>MIVSAIAANALLESVTKFHCGVIYDYSTAEYVSYRPSDFGAYLDALEAEVARGGLIVFHNGHKYDVPALTKLAKLQLNREFHLPRENCIDTLVLSRLIHSNLKDTDMGLLRSGKLPGKRFGSHALEAWGYRLGEMKGEYKDDFKRMLEEQGEEYVDGMEWWNFNEEMMDYNVQDVVVTKALLEKLLSDKHYFPPEIDFTDVGYTTFWSESLEAVDIEHRAAWLLAKQERNGFPFDTKAIEELYVELAARRSELLRKLTETFGSWYQPKGGTEMFCHPRTGKPLPKYPRIKTPKVGGIFKKPKNKAQREGREPCELDTREYVAGAPYTPVEHVVFNPSSRDH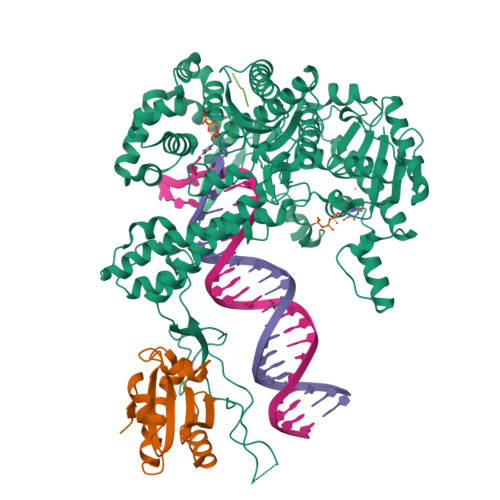IQKKLQEAGWVPTKYTDKGAPVVDDEVLEGVRVDDPEKQAAIDLIKEYLMIQKRIGQSAEGDKAWLRYVAEDGKIHGSVNPNGAVTGRATHAFPNLAQIPGVRSPYGEQCRAAFGAEHHLDGITGKPWVQAGIDASGLELRCLAHFMARFDNGEYAHEILNGDIHTKNQIAAELPTRDNAKTFIYGFLYGAGDEKIGQIVGAGKERGKELKKKFLENTPAIAALRESIQQTLVESSQWVAGEQQVKWKRRWIKGLDGRKVHVRSPHAALNTLLQSAGALICKLWIIKTEEMLVEKGLKHGWDGDFAYMAWVHDEIQVGCRTEEIAQVVIETAQEAMRWVGDHWNFRCLLDTEGKMGPNWAICH[4x];>[4x]MSDKIIHLTDDSFDTDVLKADGAILVDFWAEWCGPCKMIAPILDEIADEYQGKLTVAKLNIDQNPGTAPKYGIRGIPTLLLFKNGEVAATKVGALSKGQLKEFLDANLA;>[2x]DTDF;> TDF> GPGSMAPNTSETPANGESGPDALVEQRGHTLIVTMNRPSRRNALSGEMMQIMVEAWDRVDNDPDIRCCILTGAGGYFCAGMDLKAATKKPPGDSFKDGSYDPSRIDALLKGRRLKKPLIAAVEGPAIAGGTEILQGTDIRVAAESAKFGISEAKWSLYPMGGSAVRLVRQIPYTVACDLLL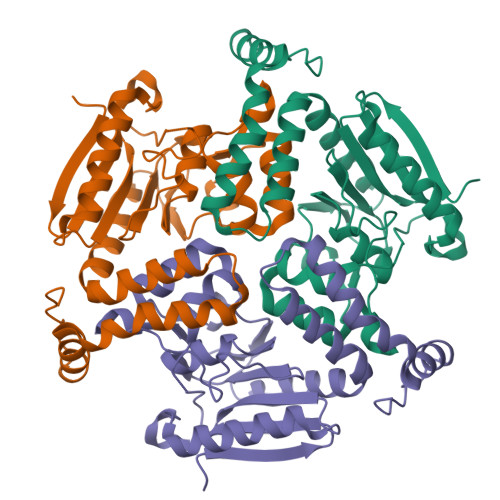TGRHITAAEAKEMGLVGHVVPDGQALTKALEIAEIIAANGPLAVQAILRTIRETEGMHENEAFKIDTRIGIEVFLSDDAKEGPQAFAQKRKPNFQNR> AAKGGDVKAASGFNAAEDAQTLRKAMKGLGTDEDAIINVLAYRSTAQRQEIRTAYKTTIGRDLMDDLKSELSGNFEQVILGMMTPTVLYDVQELRKAMKGAGTDEGCLIEILASRTPEEIRRINQTYQLQYGRSLEDDIRSDTSFMFQRVLVSLSAGGRDESNYLDDALMRQDAQDLYEAGEKKWGTDEVKFLTVLCSRNRNHLLHVFDEYKRIAQKDIEQSIKSETSGSFEDALLAIVKCMRNKSAYFAERLYKSMKGLGTDDDTLIRVMVSRAEIDMLDIRANFKRLYGKSLYSFIKGDTSGD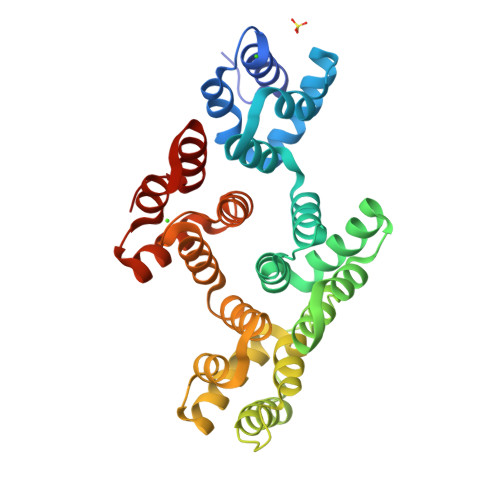YRKVLLILCGGDD> GLGDELEEVIVEKTKQTVASISSGPKHTQKVPILTANETGATMPVLPSDSIETRTTYMHFNGSETDVECFLGRAACVHVTEIQNKDATGIDNHREAKLFNDWKINLSSLVQLRKKLELFTYVRFDSEYTILATASQPDSANYSSNLVVQAMYVPPGAPNPKEWDDYTWQSASNPSVFFKVGDTSRFSVPYVGLASAYNCF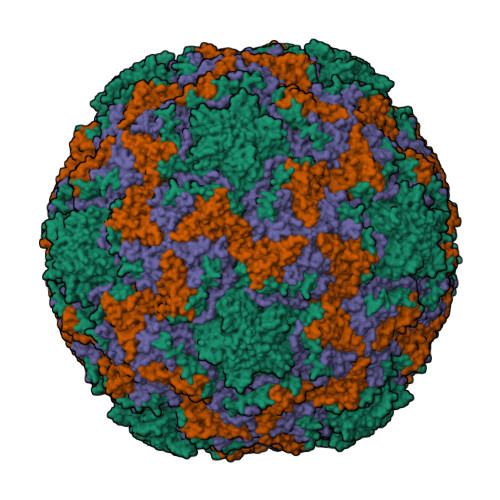YDGYSHDDAETQYGITVLNHMGGMAFRIVNEHDEHKTLVKIRVYHRAKHVEAWIPRAPRALPYTSIGRTNYPKNTEPVIKKRKGDIKSY;> SPNVEACGYSDRVQQITLGNSTITTQEAANAVVCYAEWPEYLPDVDASDVNKTSKPDTSVCRFYTLDSKTWTTGSKGWCWKLPDALKDMGVFGQNMFFHSLGRSGYTVHVQCNATKFHSGCLLVVVIPEHQLASHEGGNVSVKYTFTHPGERGIDLSSANEVGGPVKDVLYNMNGTLLGNLLIFPHQFINLRTNNTATIVIPYINSVPIDSMTRHNNVSLMVIPIAPLTVPTGATPSLPITVTIAPMCTEFSGIRSKSIVPQ;> GLPTTTLPGSGQFLTTDDRQSPSALPNYEPTPRIHIPGKVHNLLEIIQVDTLIPMNNTHTKDEVNSYLIPLNANRQNEQVFGTNLFIGDGVFKTTLLGEIVQYYTHWSGSLRFSLMYTGPALSSAKLILAYTPPGARGPQDRREAMLGTHVVWDIGLQSTIVMTIPWTSGVQFRYTDPDTYTSAGFLSCWYQTSLILPPETTGQVYLLSFISACPDFKLRLMKDTQTISQTVALTE;> GAQVSTQKSGSHENQNILTNGSNQTFTVINYYKDAASTSSAGQSLSMDPSKFTEPVKDLMLKGAPALN> ALMITDECINCDVCEPECPNGAISQGDETYVIEPSLCTECVGHYETSQCVEVCPVDAIIKDPSHEETEDELRAKYER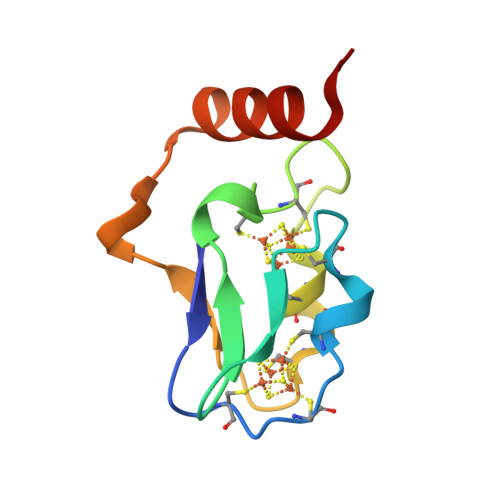ITGEG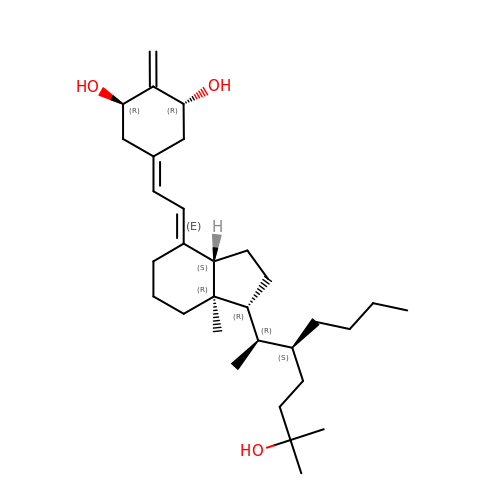(1R,3R,7E,17beta)-17-[(2R,3S)-3-butyl-6-hydroxy-6-methylheptan-2-yl]-2-methylidene-9,10-secoestra-5,7-diene-1,3-diol | C31 H52 O3 | RSXHMKSDJHHTDU-VWOHJUMJSA-N Jasmonates are phytohormones that are pivotal in mediating plant responses to various biotic and abiotic stresses and regulating plant growth. The first crystal structure of OPR3 from tomato (SlOPR3) showed that the enzyme crystallized as a self-inhibitory dimer in which the L6 loop, a critical loop involved in substrate recognition and coenzyme binding, from each protomer intrudes into the active site cavity of the other protomer. Based on these observations, it was postulated that the formation of the self-inhibitory homodimer represents a mechanism for regulating OPR3 activity and, thereby, jasmonic acid biosynthesis.

Variant Y364P was produced to test whether residue Y364 is required for homodimerization, as proposed previously. Even variant Y364P, lacking the putative phosphorylation site, was crystallized as a self-inhibitory homodimer, indicating that Y364 is not required for dimerization. The slight difference between the dimers arises from the protomers being differently positioned to each other. The sulfate binding sites (R343, Y364/P364, and R366) are the same in both dimers, and despite Y364 being replaced by a proline in Y364P, one protomer in Y364P has a bound sulfate ion at the same position as the wild type, indicating that R343 and R366 are the main binders of the sulfate ion. In the other protomer of Y364P, no sulfate ion is bound. We previously demonstrated that this sulfate binding site is instead a coenzyme-phosphate binding site responsible for NADPH binding and the enzyme's preference for NADPH over NADH10. Thus, it seems unlikely that reverse phosphorylation of Y364 serves as a regulation mechanism in vivo.

>[2x]HHHHHHMASSAQDGNNPLFSPYKMGKFNLSHRVVLAPMTRCRALNNIPQAALGEYYEQRATAGGFLITEGTMISPTSAGFPHVPGIFTKEQVREWKKIVDVVHAKGAVIFCQLWHVGRASHEVYQPAGAAPISSTEKPISNRWRILMPDGTHGIYPKPRAIGTYEISQVVEDYRRSALNAIEAGFDGIEIHGAHGYLIDQFLKDGINDRTDEYGGSLANRCKFITQVVQAVVSAIGADRVGVRVSPAIDHLDAMDSNPLSLGLAVVERLNKIQLHSGSKLAYLHVTQPRYVAYGQTEAGRLGSEEEEARLMRTLRNAYQGTFICSGGYTRELGIEAVAQGDADLVSYGRLFISNPDLVMRIKLNAPLNKPNRKTFYTQDPVVGYTDYPFLQGNGSNGPLSRL S-ETHYL-N-[4-(TRIFLUOROMETHYL)PHENYL]ISOTHIOUREA 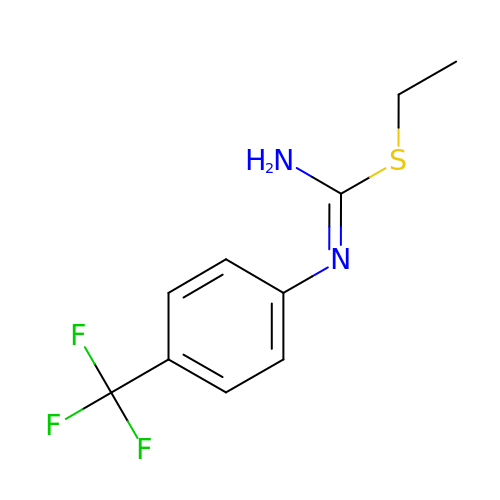| C10 H11 F3 N2 S | LCMOXIFARISMOH-UHFFFAOYSA-N>MKEVVIASAVRTAIGSYGKSLKDVPAVDLGATAIKEAVKKAGIKPEDVNEVILGNVLQAGLGQNPARQASFKAGLPVEIPAMTINKVCGSGLRTVSLAAQIIKAGDADVIIAGGMENMSRAPYLANNARWGYRMGNAKFVDEMITDGLWDAFNDYHMGITAENIAERWNISREEQDEFALASQKKAEEAIKSGQFKDEIVPVVIKGRKGETVVDTDEHPRFGSTIEGLAKLKPAFKKDGTVTAGNASGLNDCAAVLVIMSAEKAKELGVKPLAKIVSYGSAGVDPAIMGYGPFYATKAAIEKAGWTVDELDL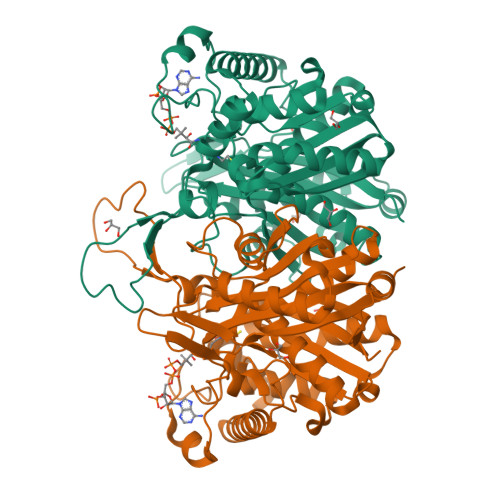IESNEAFAAQSLAVAKDLKFDMNKVNVNGGAIALGHPIGASGARILVTLVHAMQKRDAKKGLATLSIGGGQGTAILLEKCLEHHHHHH[2x]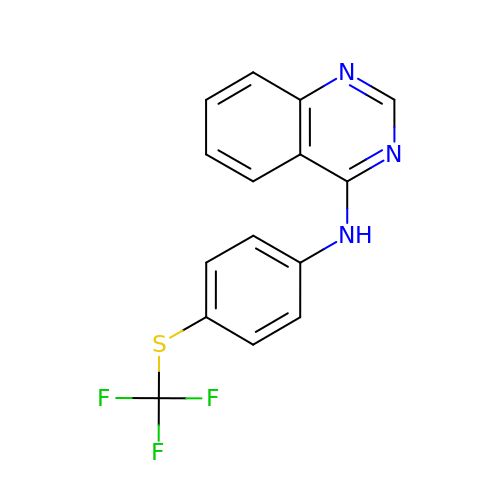N-[4-(TRIFLUOROMETHYLSULFANYL)PHENYL]QUINAZOLIN-4-AMINE | C15 H10 F3 N3 S | PZIHZHOJKADIKG-UHFFFAOYSA-N>[4x]MSVKIGINGFGRIGRLAFRRILELGEKSSDIEVVAINDLTSPALLAHLLKYDSTHGTLNADVSATDDSIVVNGKNYRVYAEPQAQ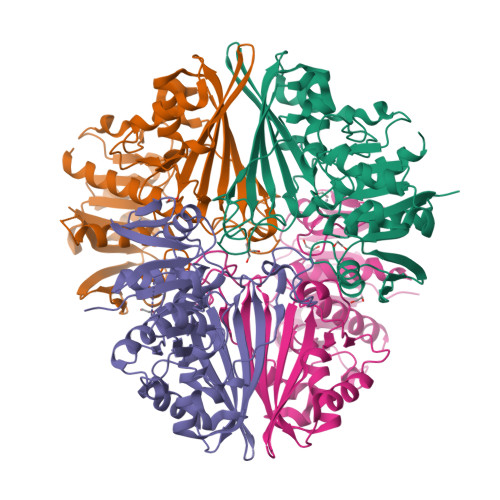NIPWVKNDGVDFVLECTGFYTSKAKSQAHLDAGAKRVLISAPAGSDLKTIVYNVNDDILTADDRIVSAGSCTTNCLAPLAFFENKEFGIKVGTMTTIHAYTSTQMLLDGPVRGGNFRAARAAGVNTIPHSTGAAKALGLVIPELNGKLQGHAQRVGVVDGSLTELVAILDKKVTADEVNAAIKKHTEGNESFGYNDDEIVSSDVIGTTFGSIFDPTQTEVTSDGDNQLVKTVAWYDNEYGFTCQMVRTLLKFATL>DLLVPKLTASVTDGAVGVTVDAPVSVTAADGVLAAVTMVNDNGRPVAGRLSPDGLRWSTTEQLGYNRRYTLNATALGLGGAATRQLTFQTSSPAHLTMPYVMPGDGEVVGVGEPVAIRFDENIADRGAAEKAIKITTNPPVEGAFYWLNNREVRWRPEHFWKPGTAVDVAVNTYGVDLGEGMFGEDNVQTHFTIGDEVIATADDNTKILTVRVNGEVVKSMPTSMGKDSTPTANGIYIVGSRYKHIIMDSSTYGVPVNSPNGYRTDVDWATQISYSGVFVHSAPWSVGAQGHTNTSHGCLNVSPSNAQWFYDHVKRGDI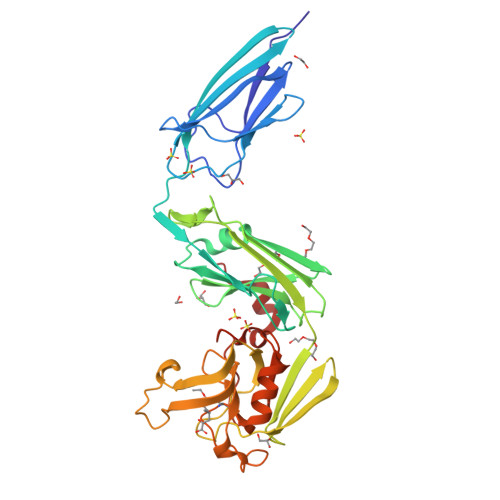VEVVNTVGGTLPGIDGLGDWNIPWDQWRAGNAKA[2x]>MRTSKKEMILRTAIDYIGEYSLETLSYDSLAEATGLSKSGLIYHFPSRHALLLGMHELLADDWDKELRDITRDPEDPLERLRAVVVTLAENVSRPELLLLIDAPSHPDFLNAWRTVNHQWIPDTDDLENDAHKRAVYLVQLAADGLFVHDYIHDDVLSKSK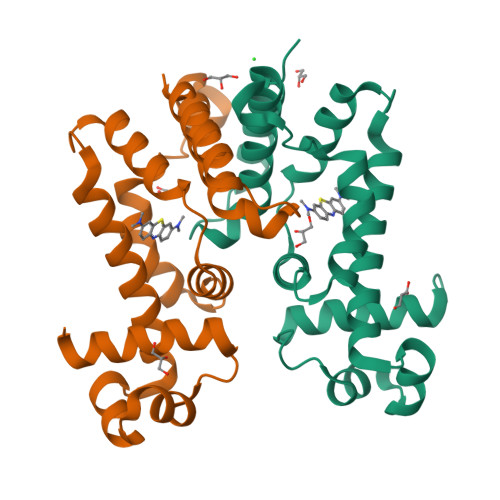RQAMLETILELIPSQTELHHHHHH[2x]>[2x]ETEAIDNGALREEAKGVFEAIPEKMTAIKQTEDNPEGVPLTAEKIELGKVLFFDPRMSSSGLISCQTCHNVGLGGVDGLPTSIGHGWQK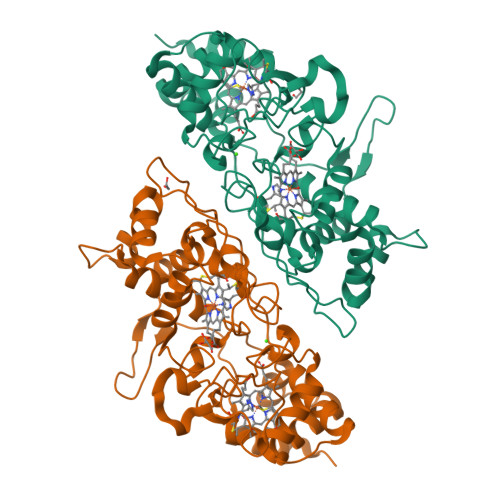GPRNAPTMLNAIFNAAQFWDGRAADLAEQAKGPVQAGVEMSNTPDQVVKTINSMPEYVEAFKAAFPEEADPVTFDNFAAAIEQFEATLITPNSAFDRFLAGDDAAMTDQEKRGLQAFMETGCTACHYGVNFGGQDYHPFGLIAKPGAEVLPAGDTGRFEVTRTTDDEYVFRAAPLRNVALTAPYFHSGVVWELAEAVKIMSSAQIGTELTDQQAEDITAFLGTLTGEQPVIDHPILPVRTGTTPLPTPM> MGAQVSSQRSGSHETGNVATGGSTINFTNINYYKDSYAASASRQDFTQDPKKFTQPVL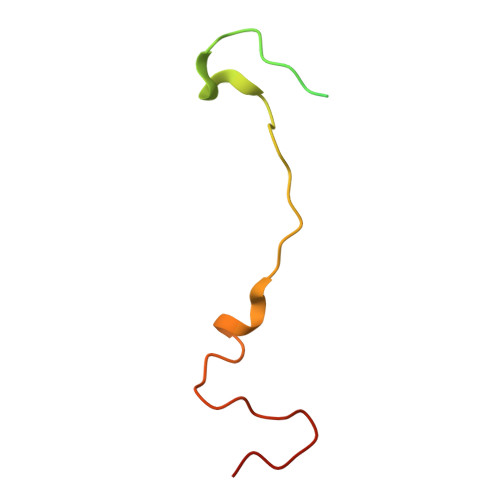DSIRELSAPLN6-oxo-2-[(2-oxo-2-phenylethyl)sulfanyl]-1,6-dihydropyrimidine-5-carboxylic acid | 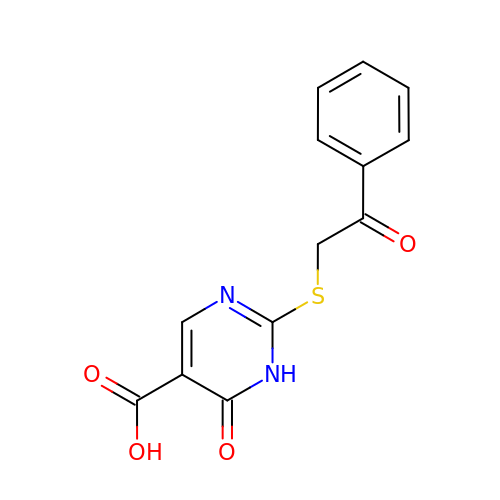C13 H10 N2 O4 S | NAHGGWKCMVAKPT-UHFFFAOYSA-N> GPDSMGA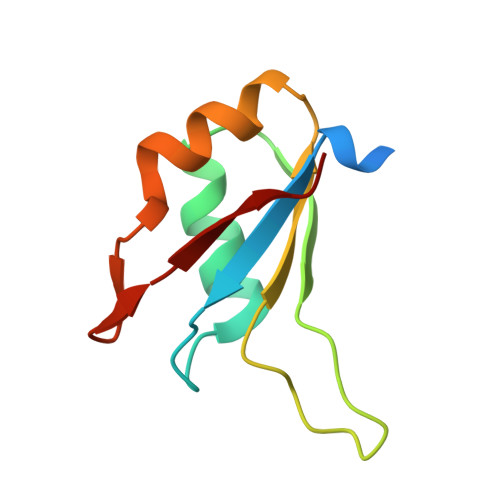AAAEADRTLFVGNLETKVTEELLFELFHQAGPVIKVKIPKDKDGKPKQFAFVNFKHEVSVPYAMNLLNGIKLYGRPIKIQFRS(1~{R},3~{S},4~{R},5~{R})-5-[(2~{S},3~{R},4~{S},5~{R})-3,4,5-tris(oxidanyl)oxan-2-yl]oxycyclohexane-1,2,3,4-tetrol 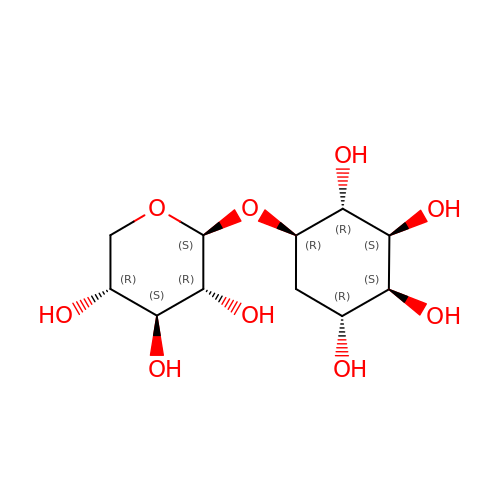| C11 H20 O9 | SGBDCDJBWZGHGQ-VBGDNJFTSA-N>[2x]GSHMSDLPLRFPYGRPEFLGLSQDEVEASADHIARPILILKETRRLPWATGYAEVINAGKSTHNEDQASCEVLTVKKKAGAVTSTPNRNSSKRRSSLPNGEGLQLKENSESEGVSCHYWSLFDGHAGSGAAVVASRLLQHHITEQLQDIVDILKNSAVLGSGSTRFFTEKKIPHECLVIGALESAFKEMDLQIERERSSYNISGGCTALI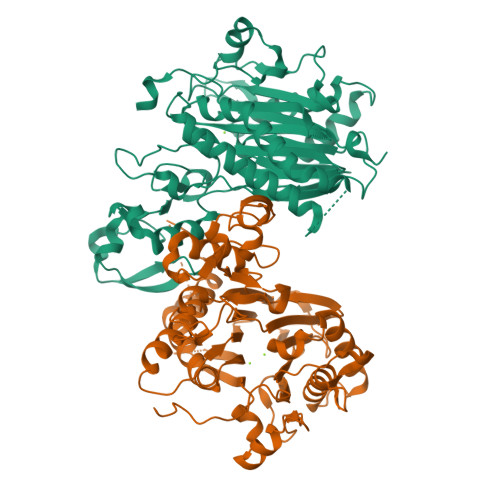VICLLGKLYVANAGDSRAIIIRNGEIIPMSSEFTPETERQRLQYLAFMQPHLLGNEFTHLEFPRRVQRKELGKKMLYRDFNMTGWAYKTIEDEDLKFPLIYGEGKKARVMATIGVTRGLGDHDLKVHDSNIYIKPFLSSAPEVRIYDLSKYDHGSDDVLILATDGLWDVLSNEEVAEAITQFLPNCDPDDPHRYTLAAQDLVMRARGVLKDRGWRISNDRLGSGDDISVYVIPLIHGNKLS Here it is shown which structural adaptations were introduced by directed evolution experiments that changed the catalytic properties of the Escherichia coli (E. coli) (S)-lactaldehyde reductase [EC 1.1.1.77]. This enzyme, referred to as FucO, is also known as an Fe2+, NAD+-dependent group-III alcohol de­hydrogenase and is involved in the catabolism of rare sugars in E. coli.

The mode of binding of NADH in the active site, including the nicotinamide moiety, is well defined by the electron density map, being the same in both structures. Also, crystal structures were obtained of the DA1472 variant in the presence of the bulky substrate analog, compound 7, cocrystallized in the presence of either NAD+ or NADH. The mode of binding of the substrate analog is the same in both structures and well defined by the electron density map. The observed mode of binding of compound 7 is possible because of the N151G and L259V amino acid changes of DA1472. In particular, the side chain of Asn151 of the wild-type active site clashes with the mode of binding of compound 7.

>MMANRMILNETAWFGRGAVGALTDEVKRRGYQKALIVTDKTLVQCGVVAKVTDKMDAAGLAWAIYDGVVPNPTITVVKEGLGVFQNSGADYLIAIGGGSPQDTCKAIGIISNNPEFADVRSLEGLSPTNKPSVPILAIPTTAGTAAEVTIGYVITDEEKRRKFVCVDPHDIPQVAFIDADMMDGMPPALKAATGVDALTHAIEGYITRGAWALTDALHIKAIEIIAGALRGSVAGDKDAGEEMALGQYVAGMGFSNVGVGLVHGMAHPLGAFYNTPHGVANAILLPHVMRYNADFTGEKYRDIARVMGVKVEGMGLEEARNAAVEAVFALNRDVGIPPHLRDVGVRKEDIPALAQAALDDVCTGGNPREATLEDIVELYHTAWTSHHHHH[2x]>[2x]MSLPMLQVALDNQTMDSAYETTRLIAEEVDIIEVG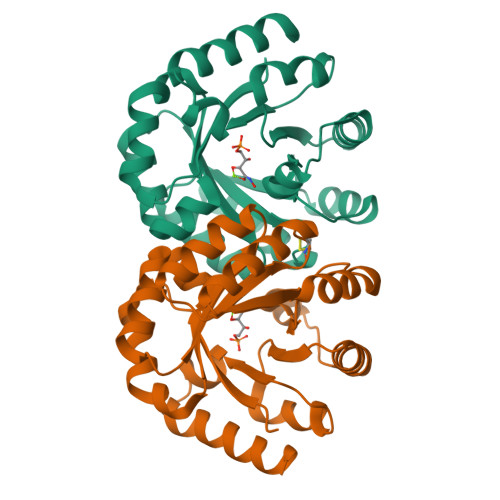TILCVGEGVRAVRDLKALYPHKIVLADAAIADAGKILSRMCFEANADWVTVICCADINTAKGALDVAKEFNGDVQIELTGYWTWEQAQQWRDAGIGQVVYHRSRDAQAAGVAWGEADITAIKRLSDMGFKVTVTGGLALEDLPLFKGIPIHVFIAGRSIRDAASPVEAARQFKRSIAELWG> QRAEEEDDDIKQ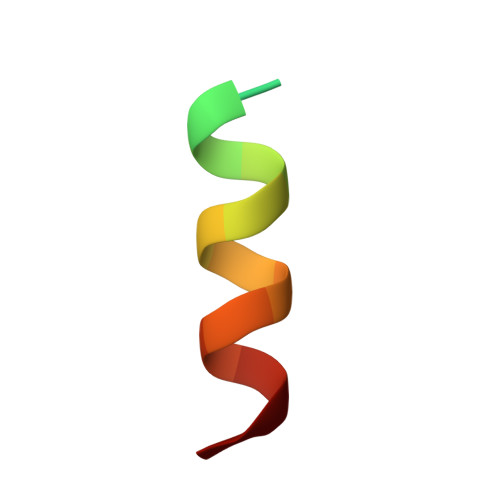LAAWAT> G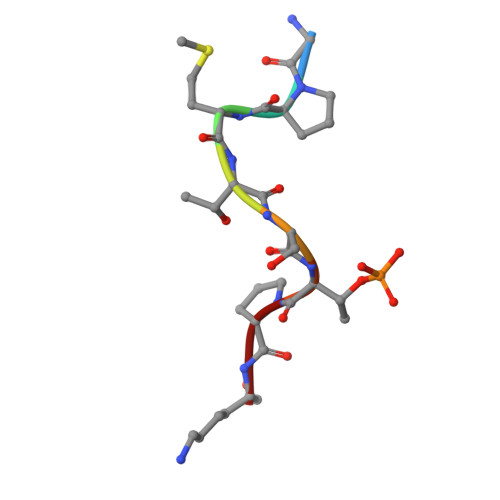PMTSTPK>[7x]SAAWEDEDLDTDNDNIPDAYEKNGYTIKDSIAVKWNDSFAEQGYKKYVSSYLESNTAGDPYTDYQKASGSIDKAIKLEARDPLVAAYPVVGVGMENLIISTNEHASSDQGKTVSRATTNSKTDANTVGVSISAGYQNGFTGNITTSYSHTTDNSTAVQDSNGESWNTGLSINKGESAYINANVRYYNTGTAPMYKVTPTTNLVLDGETLATIKAQDNQIGNNLSPNETYPKKGLSPLALNTMDQFNARLIPINYDQLKKLDSG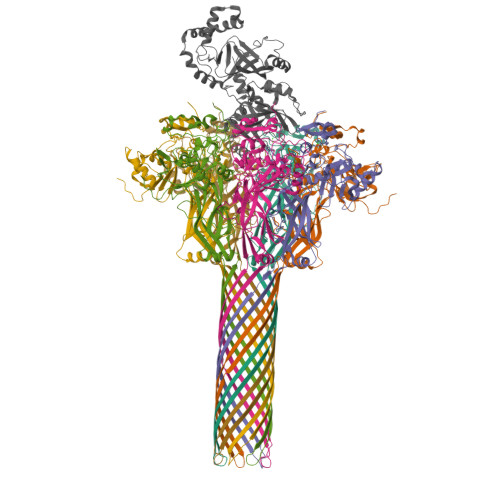KQIKLETTQVSGNYGTKNSQGQIITEGNSWSNYISQIDSVSASIILDTGSQTFERRVAAKEQGNPEDKTPEITIGEAIKKAFSATKNGELLYFNGIPIDESCVELIFDDNTSEIIKEQLKYLDDKKIYNVKLERGMNILIKVPSYFTNFDEYNNFPASWSNIDTKNQDGLQSVANKLSGETKIIIPMSKLKPYKRYVFSGYSKDPSTSNSITVNIKSKEQKTDYLVPEKDYTKFSYEFETTGKDSSDIEITLTSSGVIFLDNLSITELNSTPEILKEPEIKVPSDQEILDAHNKYYADIKLDTNTGNTYIDGIYFEPTQTNKEALDYIQKYRVEATLQYSGFKDIGTKDKEIRNYLGDQNQPKTNYINFRSYFTSGENVMTYKKLRIYAVTPDNRELLVLSVN;> GSHMAFIERPEDFLKDKENAIQWEKKEAERVEKNLDTLEKEALELYKKDSEQISNYSQTRQYFYDYQIESNPREKEYKNLRNAISKNKIDKPINVYYFESPEKFAFNKEIRTENQNEISLEKFNELKETIQDKLFKQDGFKDVSLYEPGNGDEKPTPLLIHLKLPKNTGMLPYINSNDVKTLIEQDYSIKIDKIVRIVIEGKQYIKAEASIVNSLDFKDDVSKGDLWGKENYSDWSNKLTPNELADVNDYMRGGYTAINNYLISNGPLNNPNPELDSKVNNIENALKLTPIPSNLIVYRRSGPQEFGLTLTSPEYDFNKIENIDAFKEKWEGKVITYPNFISTSIGSVNMSAFAKRKIILRINIPKDSPGAYLSAIPGYAGEYEVLLNHGSKFKINKVDSYKDGTVTKLILDATLIN>[5x]APADNAADARPVDVSVSIFINKIYGVNTLEQTYKVDGYIVAQWTGKPRKTPGDKPLIVENTQIERWINNGLWVPALEFINVVGSPDTGNKRLMLFPDGRVIYNARFLGSFSNDMDFRLFPFDRQQFVLELEPFSYNNQQLRFSDIQVYTENIDNEEIDEWWIRGKASTHISDIRYDHLSSVQPNQNEFSRITVRIDAVRNPSYYLWSFILPLGLIIAASWSVFWLESFSERLQTSFTLMLTVVAYAFYTSNILGRLPYTTYIDQMIIAGYGSIFAAILLIIFAHHRQANGVEDDLLIQRSRLAFPLGFLAIGCVLVIRFFTL

We find that reconstituting the pentameric ligand-gated ion channel (pLGIC), Erwinia ligand-gated ion channel (ELIC), in different nanodiscs produces distinct structures by cryo-EM. ELIC is one of a few pLGICs for which there is an activated, open-channel structure, and is therefore a useful structural model. Activation and opening of the channel involves a tilting of the top of M2 away from the pore axis and partial loss of the helix, such that 16′ and 9′ turn away from the pore. In the extracellular domain (ECD), ELIC activation is characterized by a counter-clockwise rotation of the ECD relative to the TMD.

We previously reported structures of ELIC in MSP1E3D1 nanodiscs with 2:1:1 lipid in the absence and presence of agonist which are resting and agonist-bound non-conducting conformations, respectively, as well as a structure of a non-desensitizing mutant, ELIC5 (P254G/C300S/V261Y/G319F/I320F), which is a putative open-channel conformation. To assess the impact of nanodiscs on the ELIC5 open-channel structure, we obtained a structure of ELIC5 with agonist in spNW15 (spNW15ELIC5) at an overall resolution of 3.4 Å. The pore-lining residues of the transmembrane helix M2, 16′ (F247) and 9′ (L240), in apo-MSP1E3D1ELIC and apo-spMSP1D1ELIC form hydrophobic constrictions consistent with a resting non-conducting conformation, while the MSP1E3D1ELIC5 and spNW15ELIC5 pores are open.>[2x]HHHHMRIEVKLLPLKDNPILPFNYNYEVYSQILEKVNSIEPTIAKLLSSPHGFWTFSRIIVRKRKILPDKGIEILSDDVSLYIS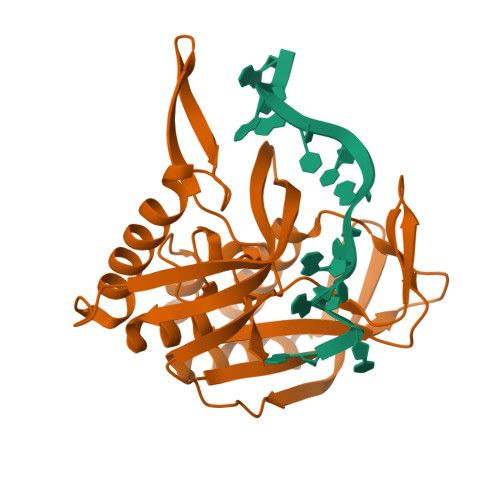SSNEDIIRAIAEAVEKSPEFKIGELSFLVGDIKAIKVKELGKENVFSTLSPIVVRTVKFEGNKLRHWDLYPHDELFMDRLRKVMILRYSEVMGETPKDRDFTIEVLKFKPTRLMVGSSYIRGSLMVFRYAGSEEIARFGYENGFGEKTGLGFGMVKLIE> MDNDGGAPPPPPTLVVEEPKKAEIRGVAFKELFRFADGLDYVLMGIGSVGAFVHGCSL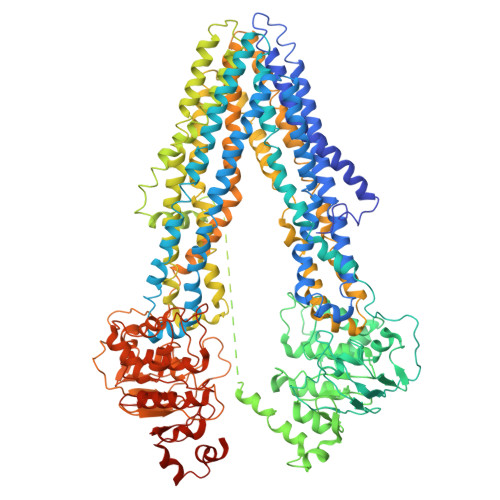PLFLRFFADLVNSFGSNSNNVEKMMEEVLKYALYFLVVGAAIWASSWAEISCWMWSGERQTTKMRIKYLEAALNQDIQFFDTEVRTSDVVFAINTDAVMVQDAISEKLGNFIHYMATFVSGFIVGFTAVWQLALVTLAVVPLIAVIGGIHTTTLSKLSNKSQESLSQAGNIVEQTVVQIRVVMAFVGESRASQAYSSALKIAQKLGYKTGLAKGMGLGATYFVVFCCYALLLWYGGYLVRHHLTNGGLAIATMFAVMIGGLALGQSAPSMAAFAKAKVAAAKIFRIIDHKPTIERNSESGVELDSVTGLVELKNVDFSYPSRPDVKILNNFCLSVPAGKTIALVGSSGSGKSTVVSLIERFYDPNSGQVLLDGQDLKTLKLRWLRQQIGLVSQEPALFATSIKENILLGRPDADQVEIEEAARVANAHSFIIKLPDGFDTQVGERGLQLSGGQKQRIAIARAMLKNPAILLLDEATSALDSESEKLVQEALDRFMIGRTTLIIAHRLSTIRKADLVAVLQQGSVSEIGTHDELFSKGENGVYAKLIKMQEAAHETAMSNARKSSARPSSARNSVSSPIMTRNSSYGRSPYSRRLSDFSTSDFSLSIDASSYPNYRNEKLAFKDQANSFWRLAKMNSPEWKYALLGSVGSVICGSLSAFFAYVLSAVLSVYYNPDHEYMIKQIDKYCYLLIGLSSAALVFNTLQHSFWDIVGENLTKRVREKMLSAVLKNEMAWFDQEENESARIAARLALDANNVRSAIGDRISVIVQNTALMLVACTAGFVLQWRLALVLVAVFPVVVAATVLQKMFMTGFSGDLEAAHAKGTQLAGEAIANVRTVAAFNSEAKIVRLYTANLEPPLKRCFWKGQIAGSGYGVAQFCLYASYALGLWYASWLVKHGISDFSKTIRVFMVLMVSANGAAETLTLAPDFIKGGQAMRSVFELLDRKTEIEPDDPDTTPVPDRLRGEVELKHIDFSYPSRPDIQIFRDLSLRARAGKTLALVGPSGCGKSSVISLIQRFYEPSSGRVMIDGKDIRKYNLKAIRKHIAIVPQEPCLFGTTIYENIAYGHECATEAEIIQAATLASAHKFISALPEGYKTYVGERGVQLSGGQKQRIAIARALVRKAEIMLLDEATSALDAESERSVQEALDQACSGRTSIVVAHRLSTIRNAHVIAVIDDGKVAEQGSHSHLLKNHPDGIYARMIQLQRFTHTQVIGMTSGSSSRVKEDDA Three capsid types have been recognized from the nuclei of herpesvirus-infected cells: empty A-capsids, scaffolding-containing B-capsids, and DNA-filled C-capsids. A unique portal vertex exists at a 12th I5 vertex through which the genome is translocated during assembly. Here, portal proteins assemble into a dodecameric basket-like structure that is thought to seed the assembly of scaffolding proteins, in turn driving the formation of spherical procapsids composed of MCP, SCP, and triplexes. A separate protein complex, the terminase, associates with the dodecameric portal and initiates genome packaging and the concurrent autoproteolytic cleavage of the scaffold.

To improve the resolution of the portal baskets, we carried out separate sub-particle reconstructions and refined them while imposing C12 symmetry, leading to portal basket structures at resolutions of 3.6, 3.5, and 3.7 Å for the A-, B-, and C-capsids, respectively. C-capsid portal baskets are positioned higher at the portal vertex compared to their A- and B-capsid counterparts, which has been attributed to the densely packed genome pushing the portal up against the capsid shell. However, our D-capsid portal structures have the same portal basket position as C-capsids despite being mostly devoid of genome. These observations together suggest that genome pressure alone does not determine portal basket height, and the elevated portal position observed in C- and D-capsids may instead be an irreversible step during capsid maturation. C-capsid portals did not vary in height but were still capable of 9 degree rotations and ~1 nm of portal basket sway. D-capsid portals had 4 Å variability in height, but otherwise resembled C-capsid portals. These findings reveal distinct patterns of portal basket variability, with A- and B-capsids exhibiting greater positional and rotational flexibility compared to the more constrained movement observed in C- and D-capsids. The C12 reconstruction of both A- and B-capsid portal baskets revealed a small hook-like density with large aromatic side chains and sharp turns wedged into a hydrophobic pocket between the crown domains of each portal monomer. This density is weaker in A-capsids, but still conspicuous, whereas it is completely absent in C-capsids, D-capsids, and mature virions (Fig. 4C through E and H through J).

>[12x]MTAPRSWAPTTRARGDTEALCSPEDGWVKVHPTPGTMLFREILHGQLGYTEGQGVYNVVRSSEATTRQLQAAIFHALLNATTYRDLEADWLGHVAARGLQPQRLVRRYRNAREADIAGVAERVFDTWRNTLRTTLLDFAHGLVACFAPGGPSGPSSFPKYIDWLTCLGLVPILRKRQEGGVTQGLRAFLKQHPLTRQLATVAEAAERAGPGFFELALAFDSTRVADYDRVYIYYNHRRGDWLVRDPISGQRGECLVLWPPLWTGDRLVFDSPVQRLFPEIVACHSLREHAHVCRLRNTASVKVLLGRKSDSERGVAGAARVVNKVLGEDDETKAGSAASRLVRLIINMKGMRHVGDINDTVRSYLDEAGGHLIDAPAVDGTLPGFGKGGNSRGSAGQDQGGRAPQLRQAFRTAVVNNINGVLEGYINNLFGTIERLRETNAGLATQLQERDRELRRATAGALERQQRAADLAAESVTGGCGSRPAGADLLRADYDIIDVSKSMDDDTYVANSFQHPYIPSYAQDLERLSRLWEHELVRCFKILCHRNNQGQETSISYSSGAIAAFVAPYFESVLRAPRVGAPITGSDVILGEEELWDAVFKKTRLQTYLTDIAALFVADVQHAALPPPPSPVGADFRPGASPRGRSRSRSPGRTAPGAPDQGGGIGHRDGRRDGRR> MLKQVEIFTDGSCLGNPGPGGYGAILRYRGREK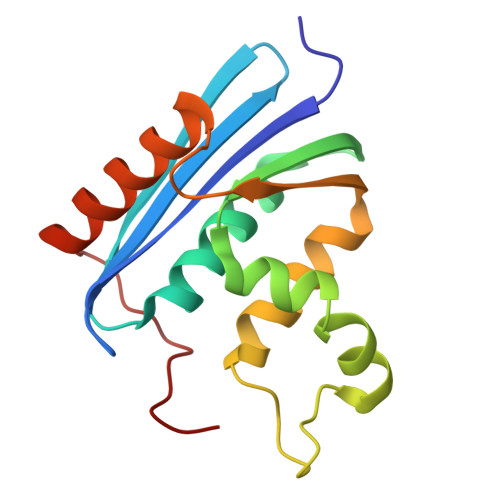TFSAGYTRTTNNRMELMAAIVALEALKEHCEVILSTDSQYVRQGITQWIHNWKKRGWKTADNKPVKNVDLWQRLDAALGQHQIKWEWVKGHAGHPENERCDELARAAAMNPTLEDTGYQVEV>GHMNKDNLRSPICCILGHVNTGKTKLLDKIRQTNVQEGEAGGITQQIGATYFPVEAIKQKTAVVNKDGKFEFKVPGLLIIDTPGHESFSNLRSRGSSLCNIAILVVDIMHGLEPQTIESLRLLRERKTPFVVALNKIDRLYGWKKIENNGFRESFALQNKAVQNEFRNRLDQVKLQFAEQGFNSELFYENKNFARYVSLVPTSAHTGEGIPDMLKLIVQLCQERMASSLMYLSELQATVLEVKAIEGFGVTIDVIL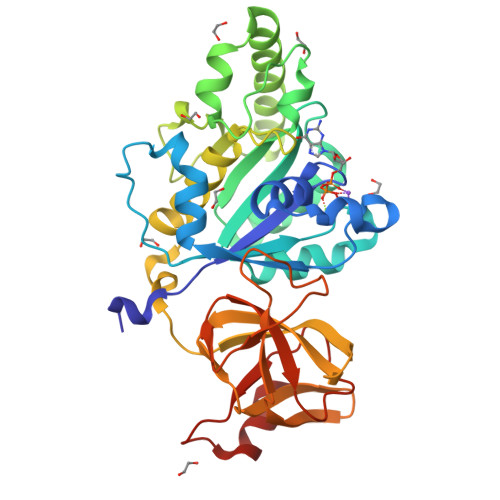SNGILREGDRIVLCGLEGPIKTNIRALLTPAPMRELRIKGQYIHHKEVKAAQGVKISAPGLEGAIAGSRLLVVGPDDDEEELEEEVESD[2x]> APITAPDITSICKDASSGIGNQEGAIRTRKCCPPSLGKKIKDFQFPNDKKVRMRWPAHKGTKKQVDDYRRAIAAMRALPDDDPRSFVSQAKIHCAYCNGGYTQVDSGFPDIDIQIH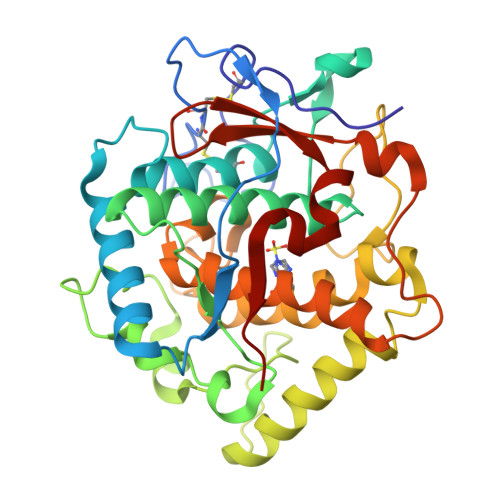NSWLFFPFHRWYLYFYERILGSLIDEPNFALPYWKWDEPKGMPISNIFLGDASNPLYDQYRDANHIEDRIVDLDYDGKDKDIPDQQQVACNLSTVYRDLVRNGVDPTSFFGGKYVAGDSPVANGDPSVGSVEAGSHTAVHRWVGDPTQPNNEDMGNFYSAGYDPVFYIHHANVDRMWKLWKELRLPGHVDITDPDWLNASYVFYDENKDLVRVYNKDCVNLDKLKYNFIENSKE> GAMGTTDDVDP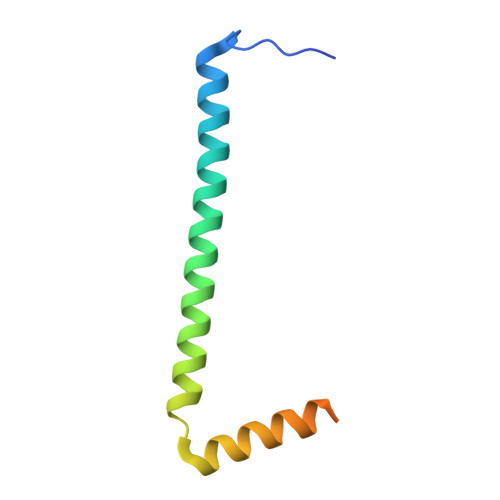EAEYAAWKLRELRRLRRERDAIEARERELAELERRRNLTEEERRAEDEAHLAKQKAEKESRGKMGYLQKYFHR>[5x]MGSSHHHHHHSSGRENLYFQGHVEEKRLSAKKGLPPGTLVYTGKYREDFEIEVMNYSIEEFREFKTTDVESVLPFRDSSTPTWINITGIHRTDVVQRVGEFFGIHPLVLEKILNVHQRPKVEFFENYVFIVLKMFTYDKNLHELESEQVSLILTKNCVLMFQE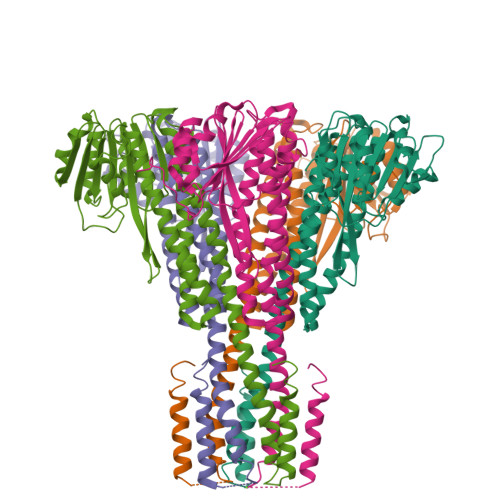KIGDVFDPVRERIRYNRGIIRKKRADYLLYSLIDALVDDYFVLLEKIDDEIDVLEEEVLERPEKETVQRTHQLKRNLVELRKTIWPLREVLSSLYRDVPPLIEKETVPYFRKVYDHTIQIADTVETFRDIVSGLLDVYLSSVSNKTNEVMKVLTIIATIFMPLTFIAGIYGMNFEYMPELRWKWGYPVVLAVMGVIAVIMVVYFKKKKWL>[10x]MIQSQINRNIRLDLADAILLSKAKKDLSFAEIADGTGLAEAFVTAALLGQQALPADAARLVGAKLDLDEDSILLL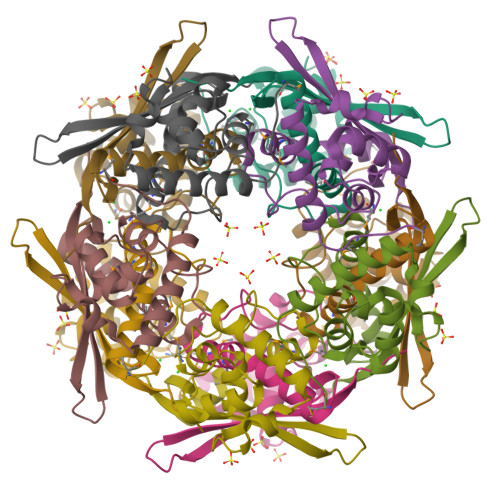QMIPLRGCIDDRIPTDPTMYRFYEMLQVYGTTLKALVHEKFGDGIISAINFKLDVKKVADPEGGERAVITLDGKYLPTKPF WbbB, a lipopolysaccharide O-antigen synthesis enzyme from Raoultella terrigena, contains an N-terminal glycosyltransferase domain with a highly modified architecture that adds a terminal β-Kdo (3-deoxy-d-manno-oct-2-ulosonic acid) residue to the O-antigen saccharide, with retention of stereochemistry. WbbB’s two C-terminal GT domains produce a polymer with a [4)-α-Rhap-(1→3)-β-GlcpNAc-(1→] repeat unit, while the N-terminal domain of the protein contains a GT99 retaining β-Kdo transferase, referred to here as WbbBGT99. Kdo addition blocks further polymerization while creating the epitope recognized by the carbohydrate-binding module of the cognate ABC transporter, allowing export prior to ligation to lipid A-core in the periplasm. The evidence presented above strongly argues that WbbBGT99 is a retaining glycosyltransferase that uses a double-displacement mechanism analogous to that used by retaining glycoside hydrolases.

We generated a WbbBGT99-D232C variant; this protein was completely labelled when expressed in BL21(DE3), but even protein expressed in ClearColiTM exhibited ~35% labelling suggesting that additional unidentified enzyme(s) with appreciable arabinose-5-phosphate isomerase activity remains active in this strain. No detectable product was found in the activity assay, implying that Cys232 cannot transfer Kdo to the acceptor. We next determined the structure of both the WbbBGT99-D232N (at 1.9 Å) and WbbBGT99-D232C (at 1.95 Å) variants as Kdo adducts. The WbbBGT99-D232C-Kdo adduct was generated by crystallizing a protein that had been spontaneously modified by the CMP-β-Kdo present during expression in E. coli BL21(DE3). In this structure, Kdo is at full occupancy, has ADPs similar to those of surrounding residues, and electron density quality comparable to that of fully buried amino acids. For both variants, clear additional density was present that could readily be modelled as an α-Kdo with an unambiguous linkage to the anomeric carbon. The Asn- and Cys- Kdo adduct structures refine with α-Kdo in a very similar position, with only small shifts (0.29 Å r.m.s.d. for Kdo compared to 0.24 Å for the protein), with the largest shifts in the anomeric carbon (0.6 Å) and carboxylate residue. The carboxylate group interacts with Arg12, as well as Ser233; in the WbbBGT99-D232N–Kdo structure, the hydrogen bond is to Ser233 N, while a ~30° rotation of the carboxylate group reorients this oxygen in the WbbBGT99-D232C–Kdo structure to instead hydrogen bond with the Ser233 Oγ. The most striking feature of the adduct structure is the dramatic reorganization of the Kdo group relative to the CMP-β-Kdo complex, with the C1 carboxylate moved furthest away from the leaving group phosphate, the exocyclic O8 group closest, and the anomeric carbon shifted 6.1 Å from the leaving group phosphate oxygen.

>MGLAVFLPPYPFRGLKAPYLWMFYKYLHCATDSILFITGEDYLSVTDDEAQRARWEFDPASMASLGYELPNAQSMACHEYLTLDNAFYETLLSRHHHDPIKSFSAFLTERIPDLETELHALLDSKKGIIDQIDTFISICNCPSLEHVARTLGKEVMHIEIGPLRAPMYRNTAYLDFAGVNGGTEASARYEKCQAEFDIKASLGDLHNYFLEVLPPAEAATHSAAGVVLQVEDCSNLIAYNHDFTNISLLSYVRQRYEKEDILVRAHPGSLFRLRDDVFTIDDSANSLAFINQCNEVFTINSSVGLEAILTGKKTTVLGDCSYAFINELAGASATVNAAAFYLFSYLVPFDLVFNQEYLKFRLGHPEEREIVGKHIEFYSADMPGSLSQAAHSLSSLINEAISLEHHHHHH[2x]>[2x]PVLVPNKEVTDGQKNINDLNVKRGDSLQYIVTGDTTELAKVDPKTVTKQGIRDTFDAEKVTIDLSKVKVYQADASLNEKDLKAVAAAINSGKAKDVTASYDLNLDQNTVTAMMKTNADGSVVLAMGYKYLLVLPF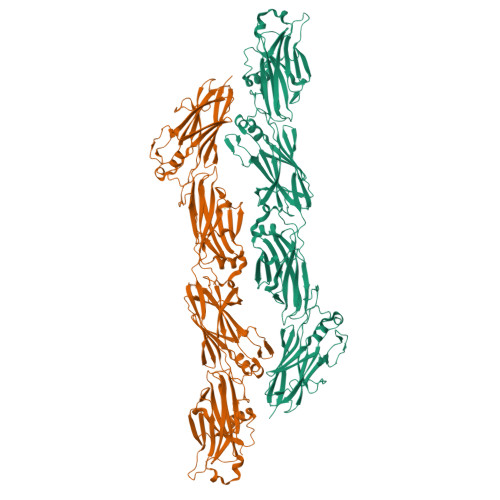VVKNVEGDFENTAVQLTNDGETVTNTVINHVPSSNPSKDVKADKNGTVGSVSLHDKDIPLQTKIYYEVKSSERPANYGGITEEWGMNDVLDTTHDRFTGKWHAITNYDLKVGDKTLKAGTDISAYILLENKDNKDLTFTMNQALLAALNEGSNKVGKQAWSVYLEVERIKTGDVENTQTENYNKELVRSNTVVTHTPDDPKPTKAVHNKKGEDINHGKVARGDVLSYEMTWDLKGYDKDFAFDTVDLATGVSFFDDYDETKVTPIKDLLRVKDSKGVDITNQFTISWDDAKGTVTISAKDPQAFILAYGGQELRVTLPTKVKADVSGDVYNSAEQNTFGQRIKTNTVVNHIPKVNPKKDVVIKVGDKQSQNGATIKLGEKFFYEFTSSDIPAEYAGVVEEWSISDKLDVKHDKFSGQWSVFANSNFVLADGTKVNKGDDISKLFTMTFDKGVVKITASQAFLDAMNLKENKNVAHSWKAFIGVERIAAGDVYNTIEESFNNEKIKTNTVVTHTPE> MLIERISDPKDLKKLLRTRNNVLVLYSKSEVAAENHLRLLSTVAQAVKGQGTICWVDCGDAESRKLCKKMKVDLSPKDKKVELFHYQD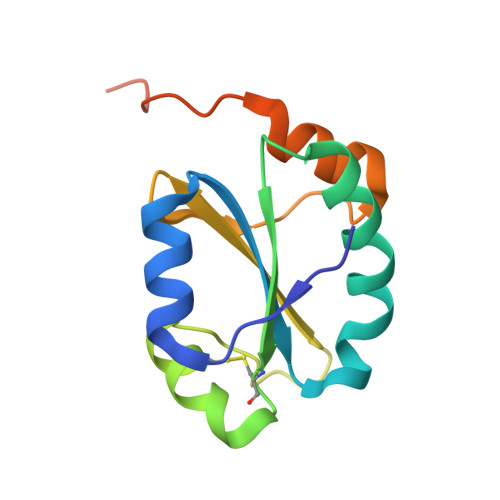GAFHTEYNRAVTFKSIVAFLKDPKGPPLWEEDPGALEHHHHHH>[3x]MKN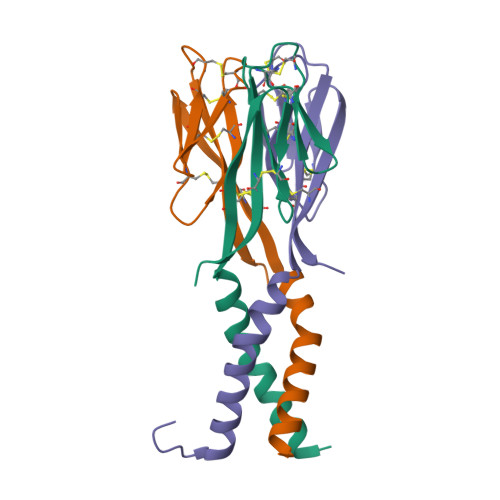LSFPLLFLFFLVPELLGSSMPLCPIDEAIDKKIKQDFNSLFPNAIKNIGLNCWTVSSRGKLASCPEGTAVLSCSCGSACGSWDIREEKVCHCQCARIDWTAARCCKLQVAS> MSLGVTQASAQWGVKASFQNYIRGSIANGSWTLNGVGFDNQQFQFSGNSGAVDAENKTGSINFPGSIHFTGHGGILDMQIANIEISFNGNSGELIADVVSSDMDGNSTNYGRTVVGTLNFSALNVSATEASGSASVSLSQSGSQAFADFYTPGTQLDPIS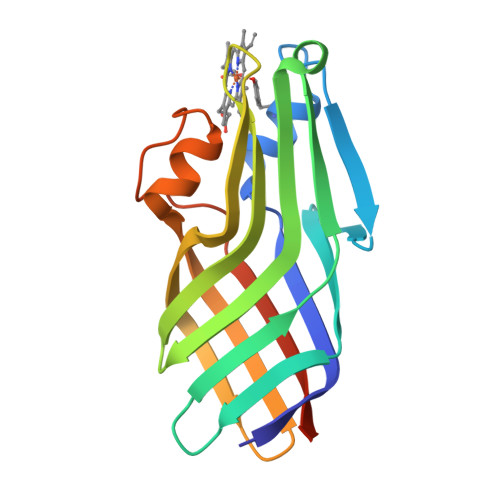FSATLGGLEHHHHHH>DIYSRLLKDRIIMLGSQIDDNVANSIVSQLLFLQAQDSEKDIYLYINSPGGSVTAGFAIYDTIQHIKPDVQTICIGMAASMGSFLLAAGAKGKRFALPNAEVMIHQPLGGAQGQATEIEIAANHILKTREKLNRILSERTGQSIEKI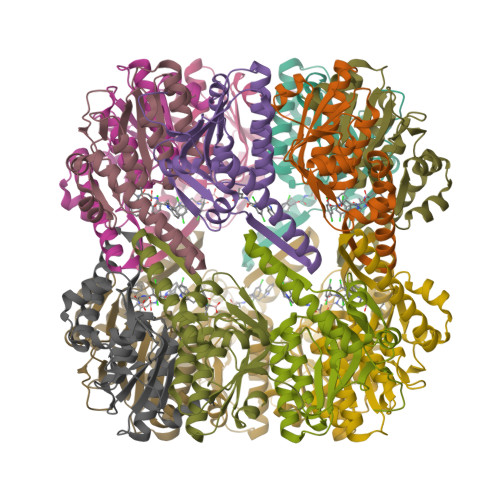QKDTDRDNFLTAEEAKEYGLIDEVMVPETK[14x]> MGEQVVKPTDERIIDPSTANTQLTGGVCYNTTSGGNKPLAGSPYGYETWIDTGGGVCSLCWYGADQGGGAAFKATWCNPHDFLGRLGYFWNENKPYSHYENIYCGFNYTRSGRKTAGDYSYIGIYGWSRNP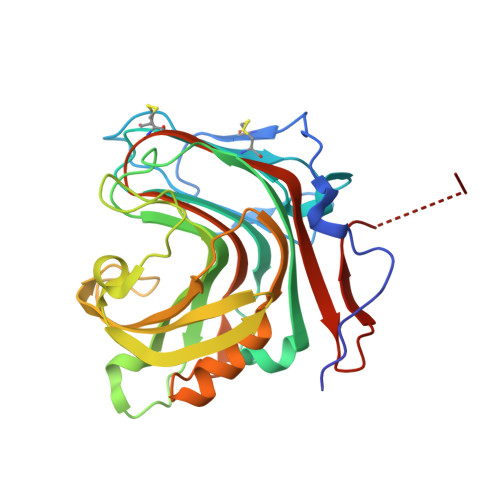SASNSNERLIEYYIVEDWFGNQWQADTSPMGINTTGGTVMGSFTVDGSSYQIIKNTRVNQPSIEGDKTFVQYFSIRQSPRKSGTISITEHFKKWEKLGMKLGDNMYECKFLIEAGAGCGFFDARLIQFYRADNEGNILQITPLEHHHHHH>MTDTIFDYVIV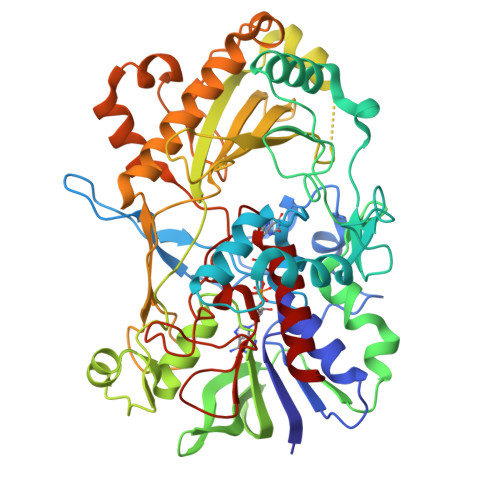GGGTAGSVLANRLSARPENRVLLIEAGIDTPENNIPPEIHDGLRPWLPRLSGDKFFWPNLTIHRAAEHPGITREPQFYEQGRLLGGGSSVNMVVSNRGLPRDYDEWQALGADGWDWQGVLPYFIKTERDADYGDDPLHGNAGPIPIGRVDSRHWSDFTVAATQALEAAGLPNIHDQNARFDDGYFPPAFTLKGEERFSAARGYLDASVRVRPNLSLWTESRVLKLLTTGNAITGVSVLRGRETLQVQAREVILTAGALQSPAILLRTGIGPAADLHALGIPVLADRPGVGRNLWEHSSIGVVAPLTEQARADASTGKAGSRHQLGIRASSGVDPATPSDLFLHIGADPVSGLASAVFWVNKPSSTGWLKLKDADPFSYPDVDFNLLSDPRDLGRLKAGLRLITHYFAAPSLAKYGLALALSRFAAPQPGGPLLNDLLQDEAALERYLRTNVGGVWHASGTARIGRADDSQAVVDKAGRVYGVTGLRVADASIMPTVPTANTNLPTLMLAEKIADAILTQA[2x]> AVKYYTLEEIQKHNNSKSTWLILHYKVYDLTKFLEEHPGGEEVLREQAGGDATENY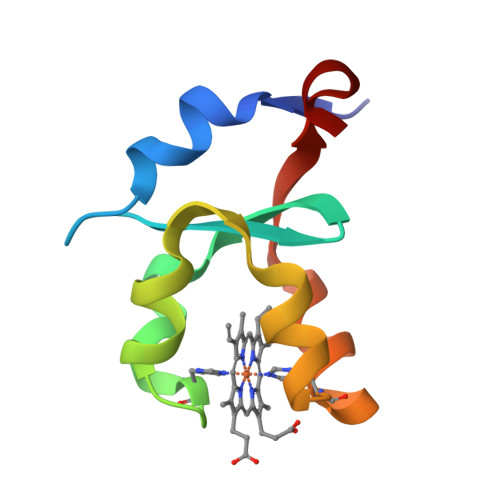EDVGHSTDARELSKTFIIGELHPDDR Recognition of viral RNAs by RLRs leads to the activation of mitochondrial antiviral signaling protein (MAVS; also known as IPS1, VISA and CARDIF). Activated MAVS triggers rapid production of type I interferons and proinflammatory cytokines. It consists of an N-terminal CARD domain, a proline-rich region (PRR) preceding a poorly structured middle segment, and a monotopic transmembrane (TM) domain at the very C-terminus. The N-terminal CARD domain of MAVS is necessary and sufficient for forming active MAVS aggregates.

To understand the structural basis underlying the filament formation, we solved the 3D structure of MAVS CARD filaments at 9.6 Å resolution by cryo-electron microscopy (cryoEM) and iterative helical real space refinement (IHRSR). The cryoEM map shows a three-stranded helical assembly with a central pore that is about 18 Å in diameter. Neighboring subunits in each strand are related by an azimuthal rotation angle (ΔΦ) of 53.6° and an axial rise (Δz) of 16.8 Å along the helical axis.Video 1. Apparent helical stripes observed in multiple filaments of different orientations suggest that the actual helical structure is left-handed. We therefore built a model of MAVS oligomer by directly fitting the crystal structure of individual MAVS CARD into the cryoEM density map (Potter et al., 2008).Video 2. Overall the MAVS CARD filament adopts a densely packed structure containing three intertwined helical strands. In the structural model of the filament, each MAVS CARD monomer directly interacts with four nearby monomers: two from the same strand and the other two respectively from two adjacent strands. The intra-strand interface makes contacts between adjacent CARDs within the same strand while the inter-strand interface holds the three strands together. At the inter-strand interface, the positive and negative charges are alternately distributed at two opposite ends of each CARD subunit, indicating that the inter-strand interaction is mainly electrostatic. The cryoEM model predicts that the intra-strand interface is stabilized mainly by hydrophobic interaction or hydrogen bonds among residues F16, W56, Y30, D53 and L48.

> MAFAEDKTYKYICRNFSNFCNVDVVEILPYLPCLTARDQDRLRATCTLSGNRDTLWHLFNTLQRRPGWVEYFIAALRGCELVDLADEVASVYQ>[3x]HHGMASMSVSTASTEMSVRKIAAHMKSNPNAKVIFMVGAGISTSCGIPDFRSPGTGLYHNLARLKLPYPEAVFDVDFFQSDPLPFYTLAKELYPGNFRPSKFHYLLKLFQDKDVLKRVYTQNIDTLERQAGVKDDLIIEAHGSFAHCHCIGCGKVYPPQVFKSKLAEHPIKDFVKCDVCGELVKPAIVFFGEDLPDSFSETWLNDSEWLREKITTS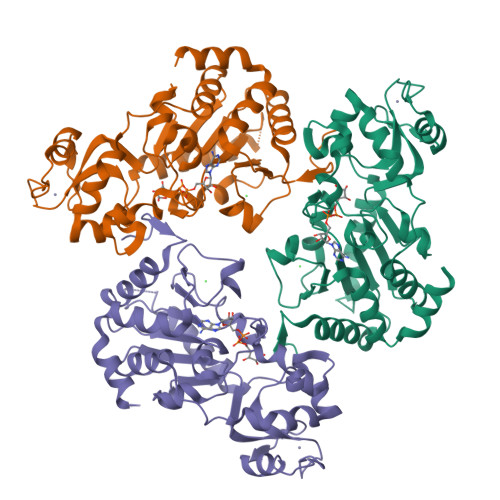GKHPQQPLVIVVGTSLAVYPFASLPEEIPRKVKRVLCNLETVGDFKANKRPTDLIVHQYSDEFAEQLVEELGWQEDFEKILTAQ>[3x]PMFIVNTNVPRASVPDGFLSELTQQLAQATGKPPQYIAVHVVPDQLMA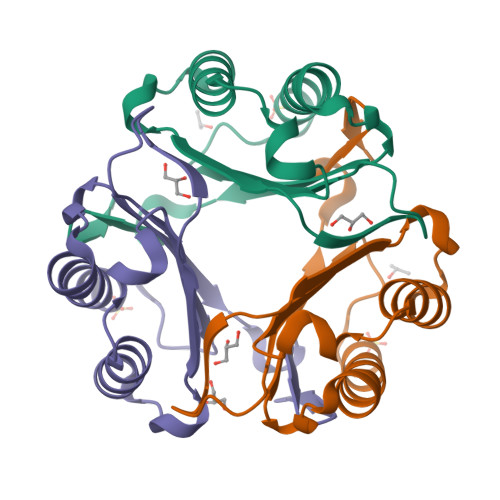FGGSSEPCALCSLHSIGKIGGAQNRSYSKLLCGLLAERLRISPDRVYINYGDMNAANVGWNNSTFA(2E)-2-(2-methoxy-2-oxoethyl)but-2-enedioic 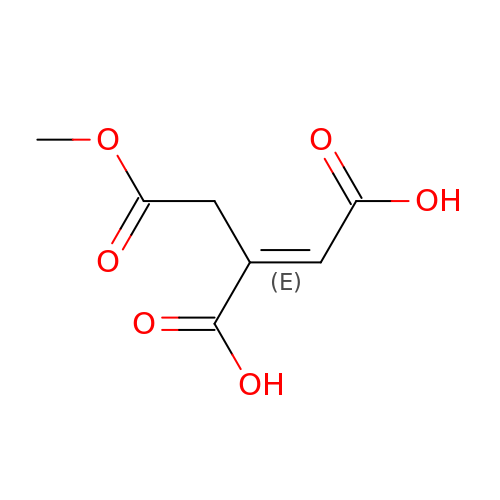acid | C7 H8 O6 | MRNZYUAGJLJQAM-DUXPYHPUSA-N>MAAGMMKDLEAFRKAQRADGPATILAIGTATPPNAVDQSSYPDYYFKITNSEHMTELKEKFRRMCDKSAIKKRYMYLTEEILKENPKVCEYMAPSLDARQDMVVVEVPRLGKEAAAKAIKEWGQPKSKITHVIFCTTSGVDMPGADYQLTKLLGLRPSVKRVMMYQQGCFAGGTVLRVAKDLAENNRGARVLVVCSEITAVTFRGPSDTHLDSMVGQALFGDGAAALIVGADPVPEVEKPCFELMWTAQTILPDSDGAIDGHLRE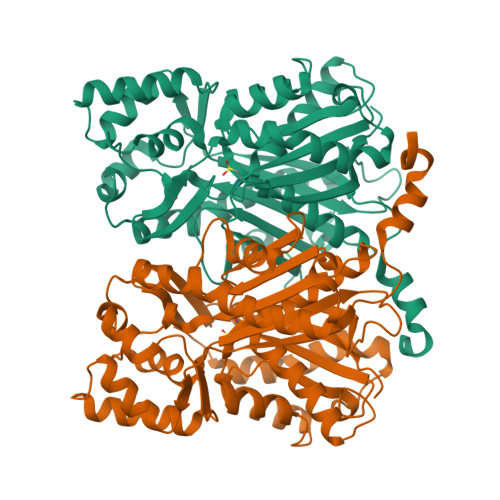VGLTFHLLKDVPGLISKNIEKSLVEAFQQFGISDWNQLFWIAHPGGPAILDQVEAKLNLDPKKLSATRQVLSDYGNMSSACVHFILDEMRKSSKEKGCSTTGEGLDVGVLFGFGPGLTVETVVLKSVPLLD[2x]>[2x]MDAPLLHIAMFPWFAMGHLTPYLHLSNKLAKRGHKISFIVPKRTQ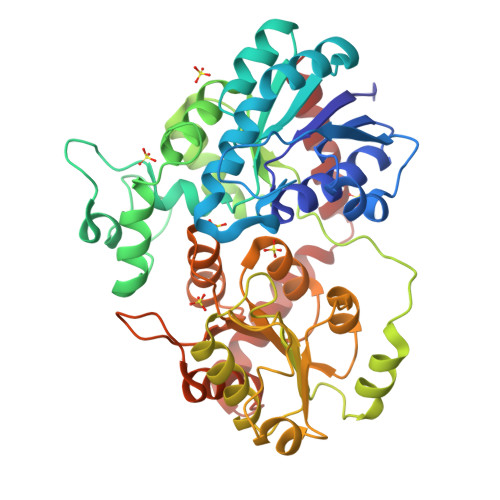TKLQHLNLHPHLITFVPITVPHIDGLPHDAETTSDVPFSLFTLIATAMDRTEKDIELLLRDLKPQIVFFDFQHWLPNLTRSLGIKSVQYLIVNPITPAYLGNRPKGRDITEADLMQPPPGFPGSAIKLHSHELRFLISTRKLEFGSGVLFLDRLSIGTRLSDAVAFKGCREIEGPYAEYLETVYGKPFLLSGPLLPEPSISTLEEKWVAWLGGFKAGSVIYCAYGSESPLQYNQFLELLLGLELTGFPFLAALKPPAGFETIEEALPEGFRERVEGRGIAYGGWVQQQMILEHPSVGCFITHCGAASITEGLVNTCQLVLLPRLGSDHIMNARLMSTKLKVGVEVEKGEEDGLFTKESVCKAVKIVMDEENEIGREVRANHTKVRNLLLSNNLESSCVDTFCDRLRGLL> MAVTDLSLTNSSLMPTLNPMIQQLAL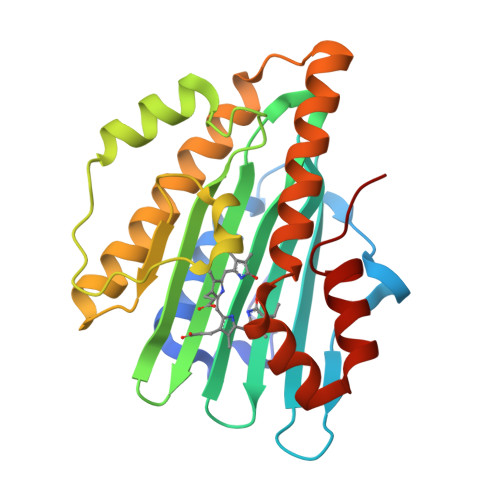AIAASWQSLPLKPYQLPEDLGYVEGRLEGEKLVIENRCYQTPQFRKMHLELAKVGKGLDILHCVMFPEPLYGLPLFGCDIVAGPGGVSAAIADLSPTQSDRQLPAAYQKSLAELGQPEFEQQRELPPWGEIFSEYCLFIRPSNVTEEERFVQRVVDFLQIHCHQSIVAEPLSEAQTLEHRQGQIHYCQQQQKNDKTRRVLEKAFGEAWAERYMSQVLFDVIQ CIS-DIBROMOETHENE | C2 H2 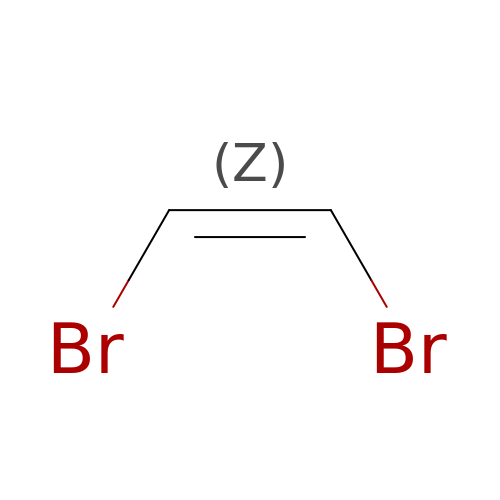Br2 | UWTUEMKLYAGTNQ-UPHRSURJSA-N>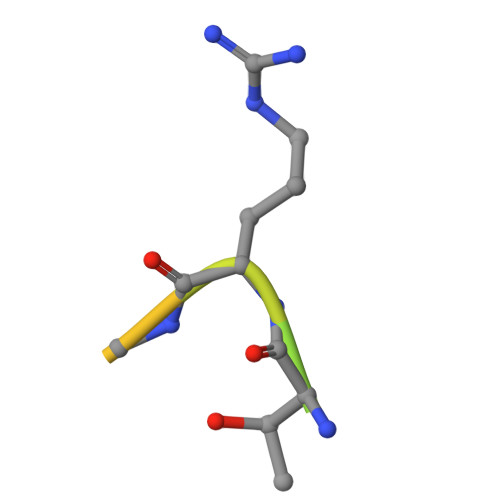 MADKPQTRSQYRNKQ> MIANVSAHRRANAFAQALEDRESEGAAAEQTETTAEPA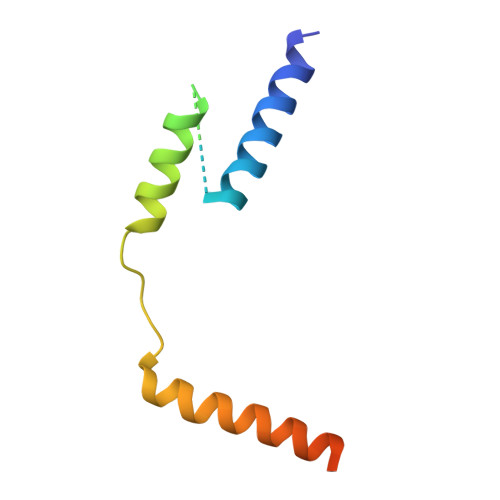EQGKLLALASGLGDLPKPQLDPEVKVVQRAQLVAAMEAMLMEGSAAAAPTVPE>[2x]TPEMPVLENRAAQGDITAPGGARRLTGDQTAALRDSLSDKPAKNIILLIGDGMGDSEITAARNYAEGAGGFFKGIDALPLTGQYTHYALNKKTGKPDYVTDSAASATAWSTGVKTYNGALGVDIHEKDHPTILEMAKAAGLATGNVSTAELQGATPAALVAHVTSRKCYGPSATSEKCPGNALEKGGKGSITEQLLNARADVTLGGGAKTFAETATAGEWQGKTLREQAEARGYQLVSDA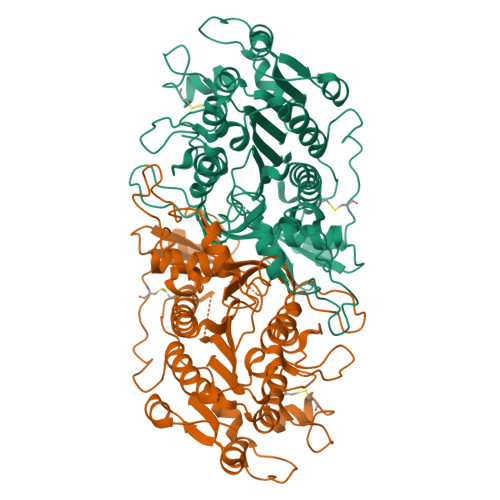ASLNSVTEANQQKPLLGLFADGNMPVRWLGPKATYHGNIDKPAVTCTPNPQRNDSVPTLAQMTDKAIELLSKNEKGFFLQVEGASIDKQDHAANPCGQIGETVDLDEAVQRALEFAKKEGNTLVIVTADHAHASQIVAPDTKAPGLTQALNTKDGAVMVMSYGNSEEDSQEHTGSQLRIAAYGPHAANVVGLTDQTDLFYTMKAALGLK> MGSSHHHHHHSSGLVPRGSHMAQAEVYSQETLAKQVLQETFGYQQFRPGQATIIDAVLEGRDCLVVMPTGGGKSLCYQIPALVKTGLTIVVSPLISLMKDQVDQLLANGVAAACLNSTQSREEQQAVLAGCRTGQVRLLYIAPERLMMDNFIDTLGYWDLAMVAVDEAH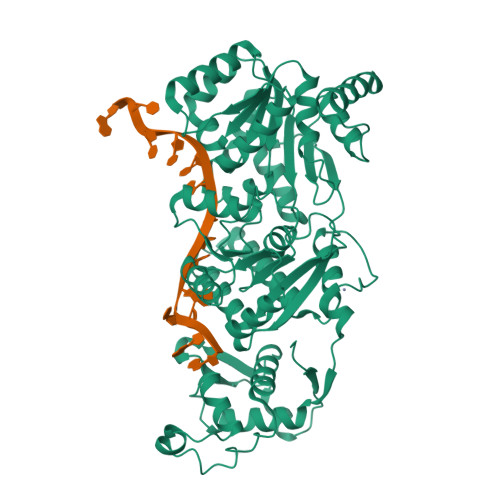CISQWGHDFRPEYAALGQLRARFPAVPFMALTATADDTTRRDIVRLLGLDDPLIEISSFDRPNIRYMLMEKFKPLDQLMRYVQEQRGKSGIIYCNSRAKVEDTAARLQSRGISAAAYHAGLEHEVRASVQEKFQRDDLQIVVATVAFGMGINKPNVRFVVHFDIPRNIESYYQETGRAGRDGLPAEAMLFYDPADMAWLRRCLEEKAPGPLQDIERHKLNAMGAFAEAQTCRRLVLLNYFGEGRQAPCGNCDICLDPPRRYDGLVDAQKALSAIARVEQRFGMGYVVEVLRGANNQRIRELGHDKLKVYGIGRDQSQEHWVSVIRQLIHLGVVTQNIAQHSALQLTEAARPFLRGEAPLMLAVPRVAALKPR>MDLAPQMLRELQETNAALQDVRELLRQQVKEITFLKNTVMECDAC[5x]

Cartilage oligomerization matrix protein (COMP) is a non-collagenous glycoprotein of the thrombospondin family that is found in cartilage, tendons, and ligaments. It is a homopentamer consisting of five subunits held together by interchain disulfide bridges in the N-terminal coiled-coil domain (COMPcc) composed of residues 27–72. The COMPcc chain fragment forms a parallel left-handed coiled-coil with an average length of 70 Å and an average outer diameter of about 30 Å. The axial pore of the pentamer is divided by the hydrophilic Gln54 ring system into two hydrophobic cavities that are exclusively lined with aliphatic side chains.

In the current work, we have solved the crystal structures of COMPcc in complex with myristic acid (C14:0), palmitic acid (C16:0), stearic acid (C18:0) and oleic acid (C18:1). In the individual COMPcc-fatty acid complex structures, one molecule of the respective fatty acid is bound inside the N-terminal hydrophobic compartment in a linear, elongated conformation. The longitudinal axis of the fatty acids are parallel to the five-fold channel symmetry. The fatty acids are retained in the binding pocket through (i) the electrostatic interaction between the electronegative carboxylate head group and the elaborate hydrogen bonding network formed by the Gln54 ring and (ii) the hydrophobic interaction existing between the aliphatic tail of the fatty acids and the hydrophobic cavities that exists between Leu37 and Leu51 residues of COMPcc. The terminal methyl groups are held in a fixed position by Thr40 (for C14:0), Leu37-Thr40 (for C16:0) and Leu37 (for C18:0). For elongated, saturated fatty acids, progressively increasing the chain length from C14 to C18 resulted in a decrease in the kd value, indicating stronger binding of the fatty acid to the channel. For example, the binding data indicate that adding two carbons to myristic acid results in a decrease of ∼0.26 kcal/mol in the binding energy. Because myristic acid has 14 carbon atoms, the contribution of the hydrophobic effect (this is equivalent to removing seven or eight pairs of carbon atoms) to the binding of myristic acid to COMPcc can be roughly estimated to be between 2.1 kcal/mol and 2.4 kcal/mol. From the Kd value, the free energy of binding of myristic acid to COMPcc can be estimated to be approximately 8.4 kcal/mol. This indicates that the hydrophobic effect contributes about a fourth of the interaction energy of the fatty acid binding.>[2x]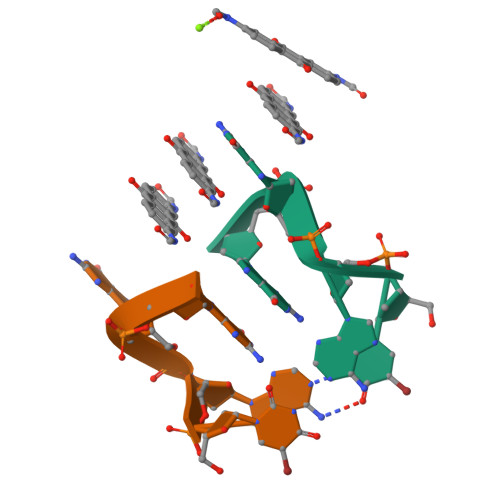UAGG>[6x]RLDPEYWKTILSCIYVFIVFGFTSFIMVIVHERVPDMQTYPPLPDIFLDSVPRIPWAFAMTEVCGMILCYIWLLVLLLHKHRSILLRRLCSLMGTVFLLRCFTMFVTSLSVPGQHLQCTGKIYGSVWEKLHRAFAIWSGFGMTLTGVHT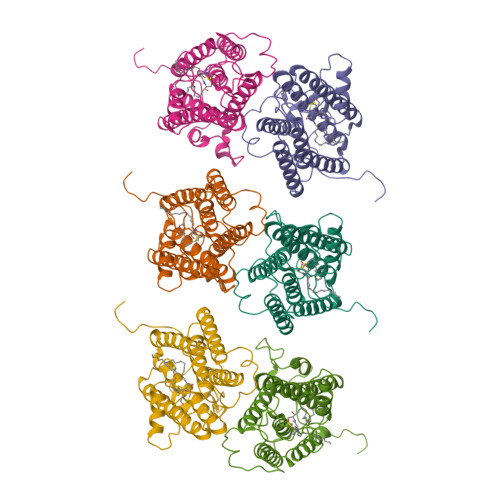CGDYMFSGHTVVLTMLNFFVTEYTPRSWNFLHTLSWVLNLFGIFFILAAHEHYSIDVFIAFYITTRLFLYYHTLANTRAYQQSRRARIWFPMFSFFECNVNGTVPNEYCWPFSKP>QHPFLNVFELERLLYTGKTACNHADEVWPGLYLGDQDMANNRRELRRLGITHVLNASHSRWRGTPEAYEGLGIRYLGVEAHDSPAFDMSIHFQTAADFIHRALSQPGGKILVHSAVGVSRSATLVLAYLMLYHHLTLVEAIKKVKDHRGIIPNRGFLRQLLALDRRLRQGLEALEH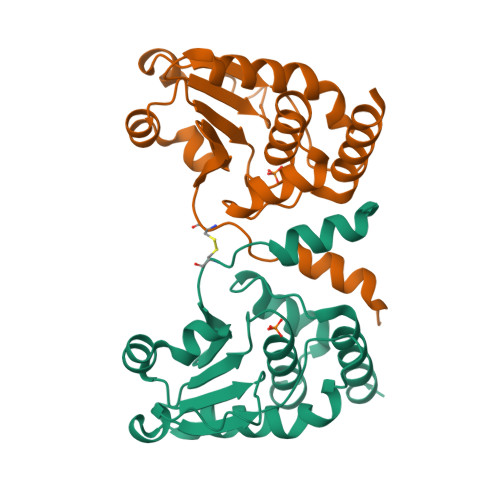HHHHH[4x]>MSLIVVTGGAGFIGSHVVDKLSESNEIVVIDNLSSGNEEFVNEAARLVKADLAADDIKDYLKGAEEVWHIAANPDVRIGAENPDEIYRNNVLATYRLLEAMRKAGVSRIVFTSTSTVYGEAKVIPTPEDYPTHPISLYGASKLACEALIESYCHTFDMQAWIYRFANVIGRRSTHGVIYDFIMKLKRNPEELEILGNGEQNKSYIYISDCVDAMLFGLRGDERVNIFNIGSEDQIKVKRIAEIVCEELGLSPRFRFTGGDRGWKGDVPVMLLSIEKL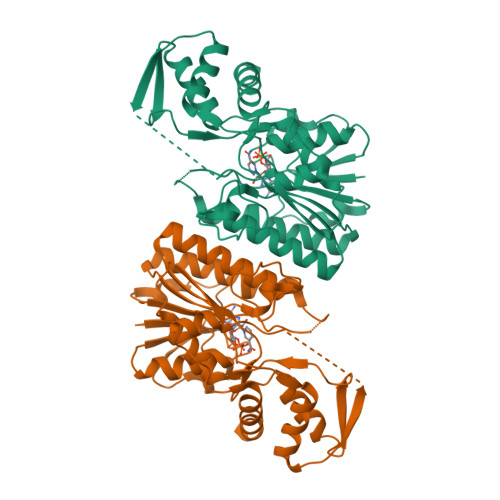KRLGWKPRYNSEEAVRMAVRDLVEDLDEEGHHHHHH[2x]> MDTNNNIEKEILALVKQNPKVSLIEYENYFSQLKYNPNASKS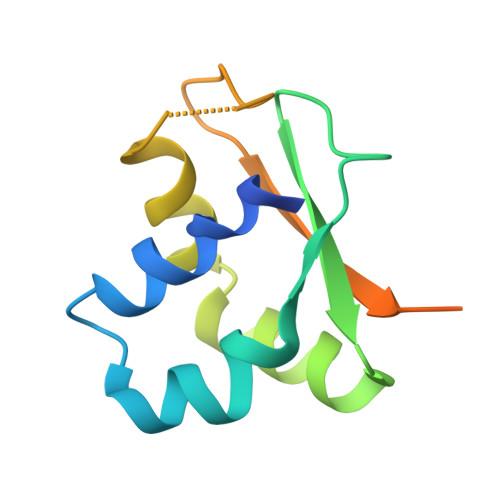DIAFFYAPNQVLCTTITAKYGALLKEILSQNKVGMHLAHSVDVRIEVAPKIQINAQSNINYKAIKTSVKD>[4x]SFVTRFTECSLSP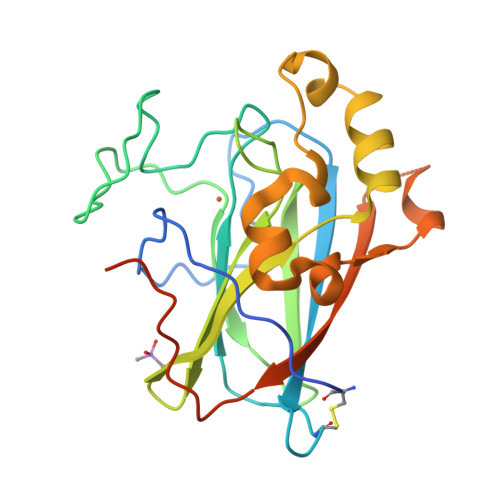EVGEGPYFIEEDIIRSNIVEDRIGIRLNVTLNLVDFNTCKPIKGAKVYIWQPDYSGIYSGFMDKPRVKREKMYPKDPRRFLRGTQVTNENGTVTFETLFPGHYPGRTPHIHYRIHANGNVAHIGQIFFDESTSQVIQSKSPYNQVHSRRMKNEEDGEFTYFNGKKSIINIDPQSLSGDSLEGILNLAINPLHRSNLMWAAGENLYFQSAGHHHHHH> GSAEAWYNLGNAYYKQGDYDEAIEYYQKALELDPRSAEAWYNLGNAYYKQGDYDEAIEYYQKAL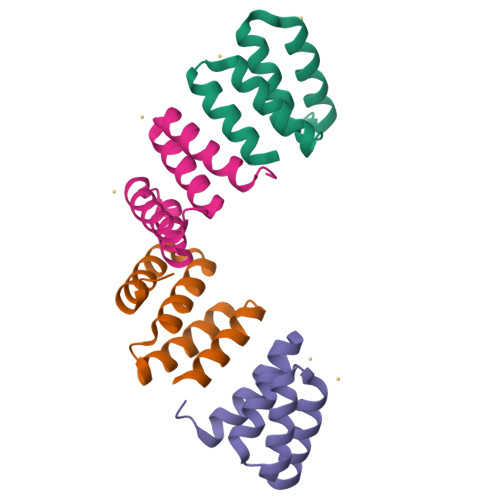ELDPRS> MQTFVHEAGRLPAHIAAELGSYRYRVFVEQLGWQLPSED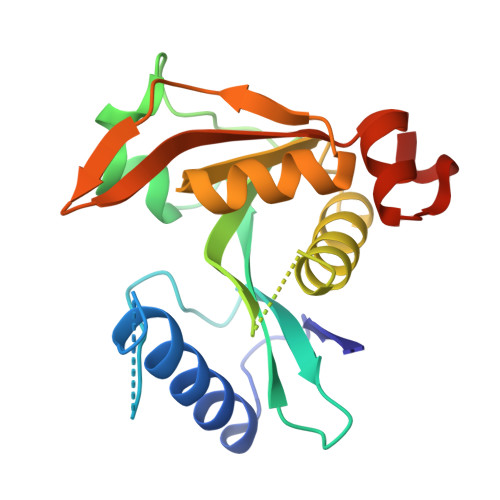EKMERDQYDRDDTVYVLGRDANGEICGCARLLPTTRPYLLQEVFPHLLADEAPRSAHVWELSRFAATPEEGADAGSLAWSVRPMLAAAVECAARRGARQLIGVTFCSMERMFRRIGVHAHRAGAPVSIDGRMVVACWIDIDAQTLAALDLDPALCASQPEAA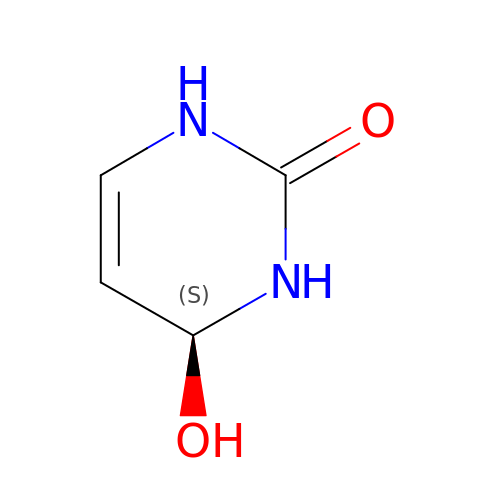4-HYDROXY-3,4-DIHYDRO-1H-PYRIMIDIN-2-ONE | C4 H6 N2 O2 | DEAAWXYGBWCVJW-VKHMYHEASA-N> LTVSARDAPTKISTLAVKVHGGSRYATKDGVAHLLNRFNFQNTNTRSALKLVRESELLGGTFKSTLDREYITLKATFLKDDLPYYVNALADVLYKTAFKPHELTESVLPAARYDYAVAEQCPVKSAEDQLYAITFRKGLGNPLLYDGVERVSLQDIKDFADKVYTKENLEVSGENVVEADLKRFVDESLLSTLPAGKSLVSKSEPKFFLGEENRVRFIGDSVAAIGIPVNKASLAQYEVLANYLTSALSELSGLISSAKLDKFTDGGLFTLFVRDQDSAVVSSNIKKIVADLKKGKDLSPAINYTKLKNAVQNESVS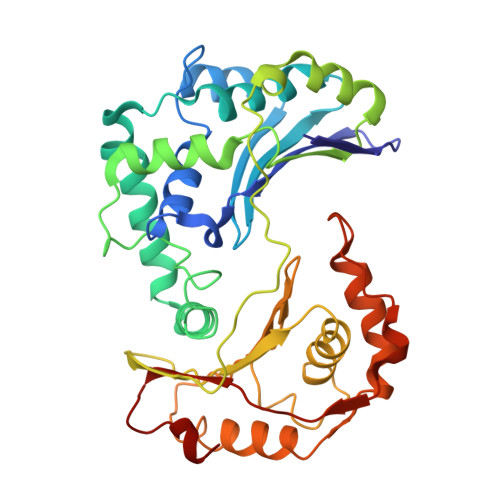SPIELNFDAVKDFKLGKFNYVAVGDVSNLPYLDEL> SGNFCPLCDKCYDDDDYESKMMQCGKCDRWVHSKCENLSDEMYEILSNLPESVAYTCVNCTERHPAEWRLALEKELQISLKQVLTA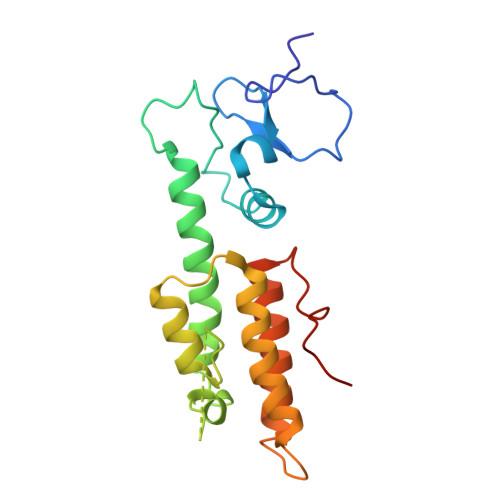LLNSRTTSHLLRYRQQQPLDLEGVKRKMDQGNYTSVLEFSDDIVKIIQAAINSDGGQPEIKKANSMVKSFFIRQMERVFPWFSVKKSRFWEPNKVSS> ASMTGGQQMGRGSSLTACPEESPLLVGPMLIEFNIPVDL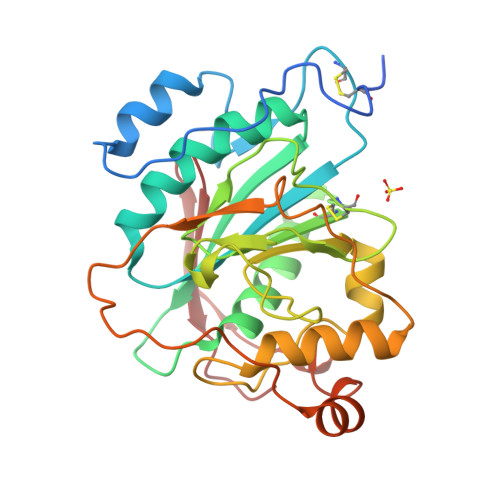KLVEQQNPKVKLGGRYTPMDCISPHKVAIIIPFRNRQEHLKYWLYYLHPILQRQQLDYGIYVINQAGESMFNRAKLLNVGFKEALKDYDYNCFVFSDVDLIPMNDHNTYRCFSQPRHISVAMDKFGFSLPYVQYFGGVSALSKQQFLSINGFPNNYWGAGGEDDDIYNRLAFRGMSVSRPNAVIGKTRMIRHSRDKKNEPNPQRFDRIAHTKETMLSDGLNSLTYMVLEVQRYPLYTKITVDIGTPS dimethyl hydrogen phosphite | C2 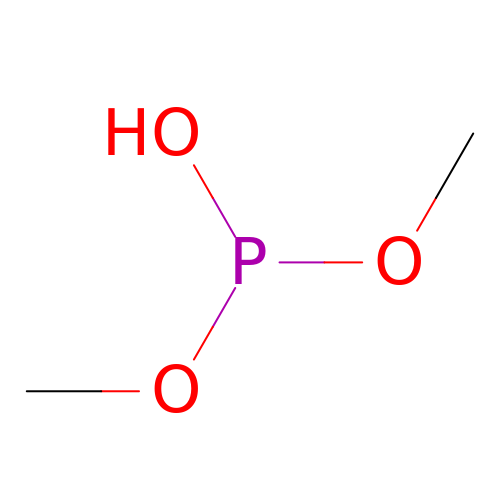H7 O3 P | DLQDGVZAEYZNTG-UHFFFAOYSA-N> MASMTGGQQMGRDPGANSGVTKNSXSPILGYWKIKGLVQPTRLLLEXLEEKYEEHLXERDEGDKWRNKKFELGLEFPNLPYXIDGDVKLTQSMAIIRXIADKHNMLGGCPKERAEISMLEGAVLDIRYGVSRIA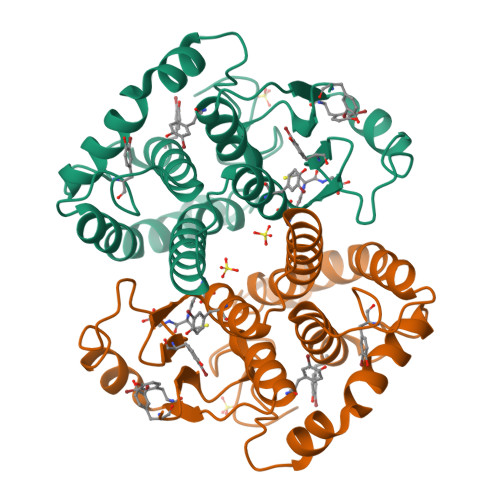YSKDFETLKVDFLSKLPEMLKMFEDRLCHKTXLNGDHVTHPDFMLYDALDVVLXMDPMCLDAFPKLVCFKKRIEAIPQIDKYLKSSKYIAWPLQGWQATFGGGDHPPKSD>MKLSELQSHIKEFDYAPEQSEHYFFKLIEEVGELSESIRKGKSGQPTLDELKGSVAEELYDVLYYVC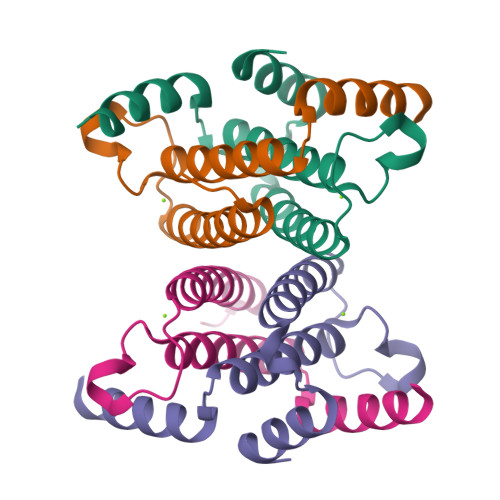ALANIHGVNLEKTHELKEVLNKVKYNRHHHHHH[4x]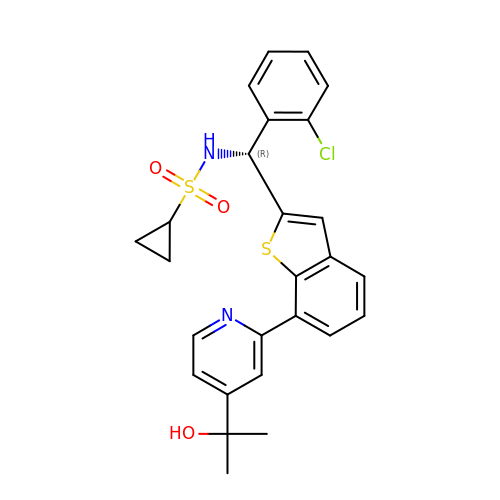N-[(R)-(2-chlorophenyl){7-[4-(2-hydroxypropan-2-yl)pyridin-2-yl]-1-benzothiophen-2-yl}methyl]cyclopropanesulfonamide | C26 H25 Cl N2 O3 S2 | CNKIRALQQHARGB-XMMPIXPASA-N[[(2~{R},3~{S},4~{R},5~{R})-5-(6-aminopurin-9-yl)-3,4-bis(oxidanyl)oxolan-2-yl]methoxy-oxidanyl-phosphoryl] 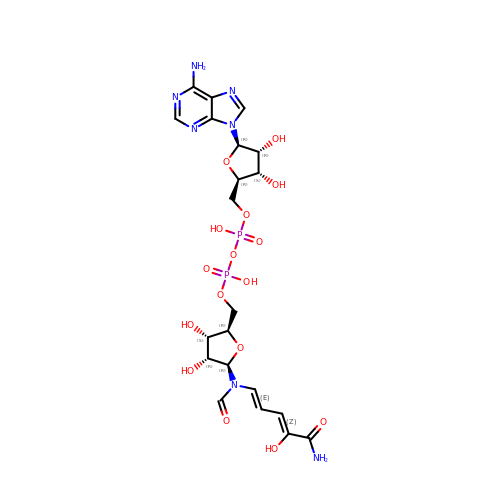[(2~{R},3~{S},4~{R},5~{R})-5-[[(1~{E},3~{Z})-5-azanyl-4-oxidanyl-5-oxidanylidene-penta-1,3-dienyl]-methanoyl-amino]-3,4-bis(oxidanyl)oxolan-2-yl]methyl hydrogen phosphate | C21 H29 N7 O16 P2 | QSTZUQWNOOUKGF-OTTADCDWSA-N2-(3,4-DIHYDRO-3-OXO-2H-BENZO[B][1,4]THIAZIN-2-YL)-N-HYDROXYACETAMIDE 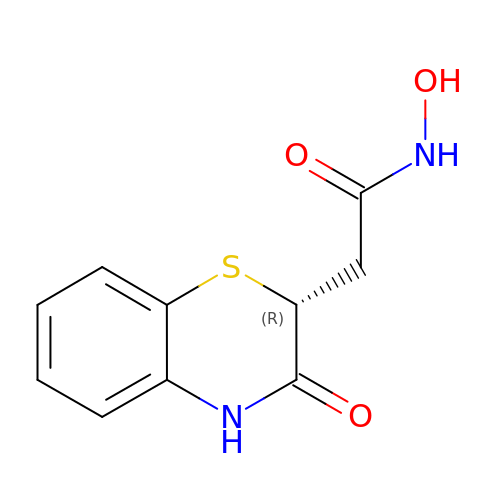| C10 H10 N2 O3 S | UKDWCJNGBPZOBU-MRVPVSSYSA-N> ERSASYKPVFVTEITDDLHFYVQDVETGTQLEKLMENMRNDIASHPPVEGSYAPRRGEFCIAKFVDGEWYRARVEK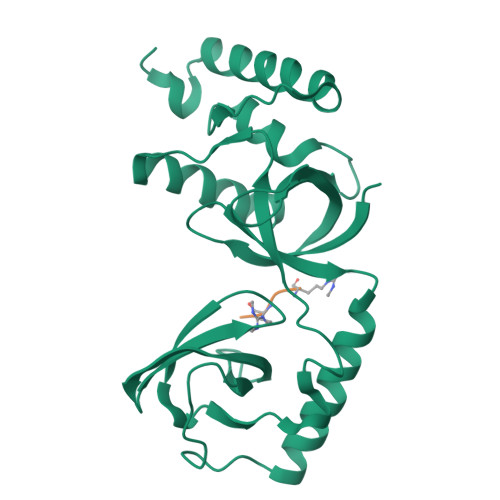VESPAKIHVFYIDYGNREVLPSTRLGTLSPAFSTRVLPAQATEYAFAFIQVPQDDDARTDAVDSVVRDIQNTQCLLNVEHLSAGCPHVTLQFADSKGDVGLGLVKEGLVMVEVRKEKQFQKVITEYLNAQESAKSARLNLWRYGDFRA;> ARGRGRHPG> GSTAPPT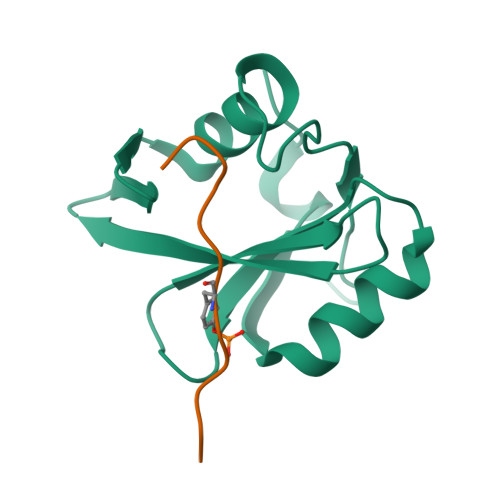NQWYHGKLDRTIAEERLRQAGKSGSYLIRESDRRPGSFVLSFLSQMNVVNHFRIIAMSGDYYIGGRRFSSLSDLIGYYSHVSSLLKGEKLLYPVAPPEPVED;> XEEENIYSVPHDST>[2x]AGKNVNVEFRKGHS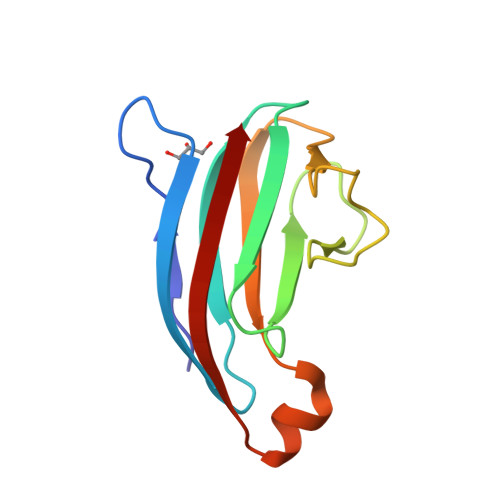SAQYSGEIKGYDYDTYTFYAKKGQKVHVSISNEGADTYLFGPGIDDSVDLSRYSPELDSHGQYSLPASGKYELRVLQTRNDARKNKTKKYNVDIQIK>ARDISIEDLLARKPKDLDDSAVAAFLKDKVVLVSGAGGTIGSELCKQCIKFGAKHLIMVDHSEYNLYKINDDLNLYKEKITPILLSILDKQSLDEVLKTYKPELILHAAAYKHVPLCEQNPHSAVINNILGTKILCDSAKENKVAKFVMISSDKAVRPTNIMGCTKRVCELYTLSMSDENFEVACVRFGNVLGSSGSVIPKFKAQIANNEPLTLTHPDIVRYFMLVAEAVQLVLQAGAIAKGGELFVLDMGKPVKIIDLAKKMLLLSNRNDLEIKITGLRKGEKLYEELL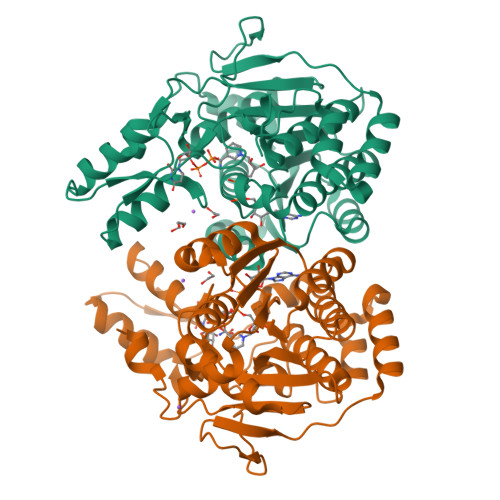IDENDAKTQYESIFVAKNEKVDLDWLNKEIENLQICEDISEALLKIVPEFKHNKEGIAAGFNRIPAAALEHHHHHH[2x]>MFPIKKRKAIKNNNINAAQIPKHIAIIMDGNGRWAKQKKMPRIKGHYEGMQTVRKITRYASDLGVKYLTLYAFSTENWSRPKDEVNYLMKLPGDFLNTFLPELIEKNVKVETIGFIDDLPDHTKKAVLEAKEKTKHNTGLTLVFALNYGGRKEIISAVQLIAERYKSGEISLDEI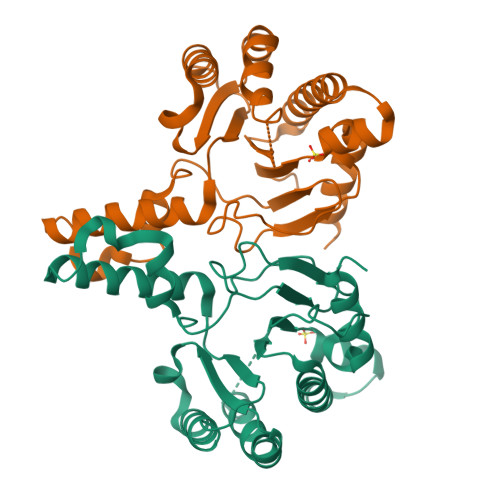SETHFNEYLFTANMPDPELLIRTSGEERLSNFLIWQCSYSEFVFIDEFWPDFNEESLAQCISIYQNRHRRFGGL[2x]>[6x]MTYVILPLEMKKGRGYVYQLEYHLIWCVKYRHQVLVGEVADGLKDILRDI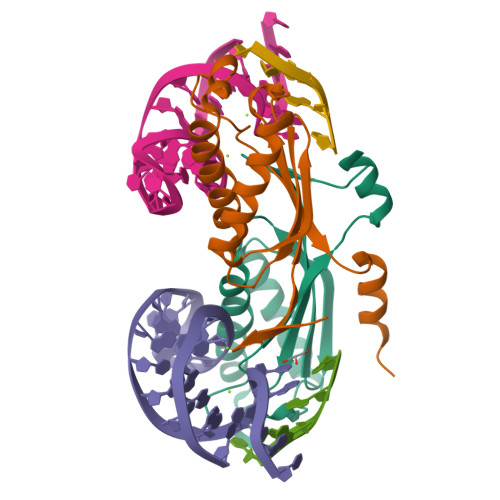AAQNGLEVITMEVMPDHVHLLLSATPQQAIPDFVKALKGASARRMFVAYPQLKEKLWGGNLWNPSYCILTVSENTRAQIQKYIESQHDKE Orn and NrnC are 3′–5′ exonucleases with a DnaQ fold containing the catalytic DEDD motif, a domain that is common in enzymes that act on nucleic acids. Notably, Orn (and its eukaryotic ortholog REXO2) or NrnC activity is critical for cellular growth, rendering them unique amongst the exoribonucleases known to date. Through quantitative structure-function analyses, we show here that NrnC-type RNases share this narrow substrate length preference with Orn. The structures confirm an octameric assembly as a conserved feature of NrnC-type RNases.

To further understand the structural basis of NrnC’s substrate preference, we determined structures of B. melitensis NrnC (NrnCBm) in several apo and partially pGG-bound states. (C) Superposition of four apo-NrnCBm conformations based on three independent crystal forms (comprising chains apo1A/apo1B for form 1; apo2A/apo2B for form 2, and apo3A/pGG-bound3B for form 3), compared to the pGG-bound conformation of the same protein shown in (B). In contrast, the Y150 side chain points away from the active site in substrate-free NrnC. While the octameric assembly remains in the absence of substrate, this loop moves outward from the active site and D113 rotates away from the substrate. The most drastic conformational change however is attributed to a flexible loop spanning residues 130SKQQQS135. In contrast, in the substrate-free state NrnCBm, captured in the mixed-state structure or a homogeneous apo-state structure, this loop swings away from the active site or is completely disordered, leading to an overall widening of the active site.

>[2x]SMTIRFHRNDLPNLDNYQVDAVAIDTETLGLNPHRDRLCVVQISPGDGTADVIQIEAGQKKAPNLVKLLKDRSITKIFHFGRFDLAVLAHAFGTMPQPVFCTKIASKLTRTYTDRHGLKEICSELLDVSISKQQQSSDWAAEVLSQAQLEYAASDVLYLHRLKAVLEQRLERDGRTKQAEACFKFLPTRSELDLMGWAESDIFAHS The peptidylarginine deiminase enzymes (PADIs, or PADs, herein referred to as PADIs) catalyse the post-translational conversion of protein arginine residues to non-coded citrulline, in a process termed citrullination or peptidylarginine deimination. PADI4 possesses a nuclear localisation sequence and targets a variety of nuclear substrates, including core and linker histones, through which it modulates gene expression and chromatin compaction. PADIs require calcium for catalysis, and the sequential binding of calcium ions results in a large structural rearrangement that forms the active site cleft. We report PADI4_3, a cell-active inhibitor specific for the active conformation of PADI4; PADI4_7, an inert binder, which we functionalise for the isolation and study of cellular PADI4; and PADI4_11, a cell-active PADI4 activator.

The lead-activating peptide, PADI4_11, lowers the calcium requirement for activation in vitro and induces activation within cells in the absence of any additional stimuli. We then used cryoEM to elucidate the mode of binding of PADI4_11 to PADI4 and were able to obtain a structure with an overall resolution of 3.6 Å. As for the structure with the inhibitor PADI4_3 described above, PADI4 adopts a homodimeric structure. PADI4_11 adopts an alpha-helical structure with the internal cyclisation bridge between C4 and the N-terminus of the peptide acting like a peptide staple. The structure revealed that PADI4_11 binds to a surface of PADI4 distal to the active site, but close to the five calcium ion binding sites. The peptide binds in a cleft formed between two loops in PADI4 (D155-V171 and P371–387). PADI4_11 binding in this region thus fits well with our observations that PADI4_11 activates PADI4 by reducing its calcium dependency, since peptide binding likely alters the dynamics of this region and may, therefore, directly increase calcium binding affinities. By contrast, substitution of E2 by alanine, aspartic acid or glutamine all resulted in loss of activity, suggesting the importance of the appropriate side chain length, as well as negative charge in position 2 of PADI4_11, in allowing it to form a salt bridge with R394 in PADI4. The structural and mutagenesis analyses presented here reveal that PADI4_11 binds at an allosteric site on PADI4, in a region of the protein that is disordered in calcium-free crystal structures but becomes structured upon calcium binding.

>[2x]GPLGSPQMAQGTLIRVTPEQPTHAVCVLGTLTQLDICSSAPDDCTSFSINASPGVVVDIAHSPPAKKKSTGSSTWPLDPGVEVTLTMKAASGSTGDQKVQISYYGPKTPPVKALLYLTAVEISLCADITRTGKVKPTRAVKDQRTWTWGPCGQGAILLVNCDRDNLESSAMDCEDDEVLDSEDLQDMSLMTLSTKTPKDFFTNHTLVLHVARSEMDKVRVFQATRGKLSSKCSVVLGPKWPSHYLMVPGGKHNMDFYVEALAFPDTDFPGLITLTISLLDTSNLELPEAVVFQDSVVFRVAPWIMTPNTQPPQEVYACSIFENEDFLKSVTTLAMKAKCKLTICPEEENMDDQWMQDEMEIGYIQAPHKTLPVVFDSPRNRGLKEFPIKRVMGPDFGYVTRGPQTGGISGLDSFGNLEVSPPVTVRGKEYPLGRILFGDSCYPSNDSRQMHQALQDFLSAQQVQAPVKLYSDWLSVGHVDEFLSFVPAPDRKGFRLLLASPRSCYKLFQEQQNEGHGEALLFEGIKKKKQQKIKNILSNKTLREHNSFVERCIDWNRELLKRELGLAESDIIDIPQLFKLKEFSKAEAFFPNMVNMLVLGKHLGIPKPFGPVINGRCCLEEKVCSLLEPLGLQCTFINDFFTYHIRHGEVHCGTNVRRKPFSFKWWNMVP;>YESCRYRQVLQLX[2x]>MRKLAIALLFPAAAVLAEPAAAPNGISLPAGYKDWKMIGVSSRIEQNNLRAILGNDIAVKAAREGRTHPWPDGAILVKLSWKKSTHELFPSAEVPGDFTQADFMVKDAAKYASTGGWGYARWLGMEQKPYGANADFAQEC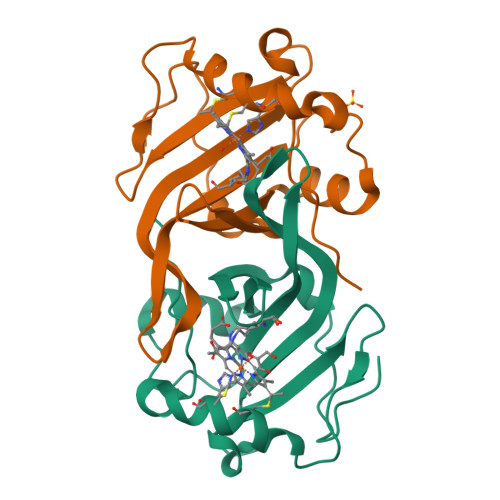MGCHSGAKAADYVFTHPAKLP[2x]>MRSRRVDVMDVMNRLILAMDLMNRDDALRVTGEVREYIDTVKIGYPLVLSEGMDIIAEFRKRFGCRIIADFKVADIPETNEKICRATFKAGADAIIVHGFPGADSVRACLNVAEEMGREVFLLTEMSHPGAEMFIQGAADEIARMGVDLGVKNYVGPSTRPERLSRLREIIGQDSFLISPGAGAQGGDPGETLRFADAIIAGRSIYLADNPAAAAAGIIE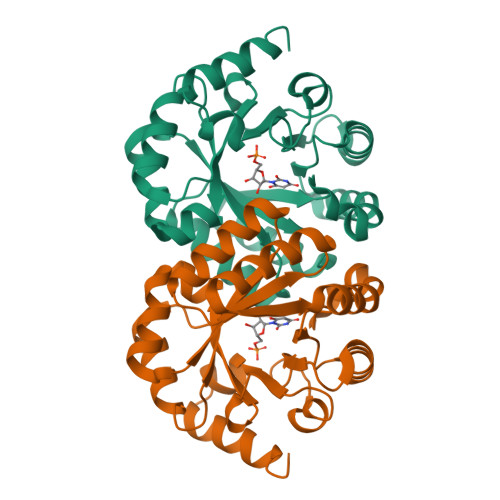SIKDLLNP[2x]>[4x]MKTLIARHKAGEHIGICSVCSAHPLVIEAALAFDRNSTRKVLIEATSNQVNQFGGYTGMTPADFREFVFAIADKVGFARERIILGGDHLGPNCWQQENVDAAMEKSVELVKAYVRAGFSKIHLDASMSCAGDPIPLAPETVAERAAVLCFAAESVATDCQREQLSYVIGTEVPVPGGEASAI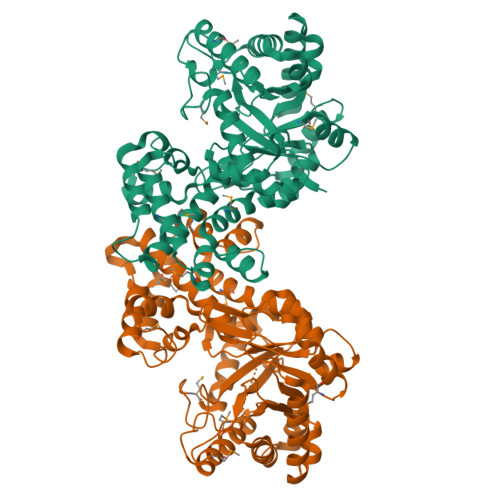QSVHITHVEDAANTLRTHQKAFIARGLTEALTRVIAIVVQPGVEFDHSNIIHYQPQEAQALAQWIENTRMVYEAHSTDYQTRTAYWELVRDHFAILKVGPALTFALREAIFALAQIEQELIAPENRSGCLAVIEEVMLDEPQYWKKYYRTGFNDSLLDIRYSLSDRIRYYWPHSRIKNSVETMMVNLQGVDIPLGMISQYLPKQFERIQSGELSAIPHQLIMDKIYDVLRAYRYGCAE>[5x]NRQLERSGRFGG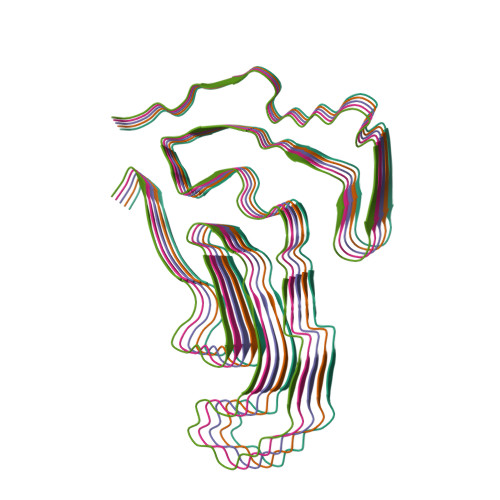NPGGFGNQGGFGNSRGGGAGLGNNQGSNMGGGMNFGAFSINPAMMAAAQAALQSSWGMMGMLASQQNQSGPSGNNQNQGNMQREPNQAFGSGNNSYSGSNSGAAIGWGSASNAGSGSGFNGGFGSSMDSKSSGWGM>MPSYLSPGVYVEEVASGSRPIEGVGIEGVGTSVAAFVGLAPTGPLNEPTLVTNWTQYVAAFGDFTGGYYLAHSVYGFFNNGGSAAYVVRVGGSAEDAAADGSVNGAAAPAAVTGSTAKALPAAEPKQLGTFAVTATAAGQSGPLTVEVADPEGEGPAERFKLIVKDGDKPVETFDVSAKKGNRSYVVTQVKERSKLITVTEAAPSAQLVRPENQSLTLPAPPSAAPAVPAGQAESAHPGPAQYLGDSSDRTGFGGLEAIDEISMVAVPDLMAAYQRGAIDLEAVKAVQLGLIAHCELMGDRVAIIDPPPNQNARQIRVWRQETAGYDSKYAALYYPWIKSFDPATGQSRLVPPSGHVAGIWARNDSERGVHKAPANEVVRGAVDLELQITRGEQDLLNPIGVNCIRSFPGRGIRVWGARTLSSDPAWRYLNIRRYFNYLEESILIGTQWVVFEPNDHNLWARIRRNVSAFLVNEWRNGALFGQSPDQAYYVKCDEETNPPESVDLGRVVCEIGIAPVKPAEFVIFRLAQFSSGGGELDE[24x];>[24x]MSLPKPEDVLVAPNFGIQIDGVMVEYLNSVSNLQIEQDVIRYQQNQGTTGRNNVTLMPGVAKDGSVQVERGMSQSSVFTQWINDSMAGRMATARKNATIIVMDYEDNPVKRWNLRNAWCSKVVAGTLKAGDTNALTETITIVFEELVVE

In general, CIS are composed of a contractile sheath that surrounds an inner tube loaded with effectors, fitted with a baseplate complex. A conformational change in the baseplate complex triggers the contraction of the outer sheath, which leads to the propulsion of the inner tube into the target. Here we provide evidence that CIS from the model organism Streptomyces coelicolor (CISSc) function intracellularly and belong to a new class of CIS that exist as free-floating fully assembled particles in the cytoplasm and mediate cell death in response to stress conditions. Similar to the recently described sheath structures observed in AlgoCIS15 and tCIS19, the CISSc sheath is composed of a single protein, Cis2.

Different sets of two (IE), three (IEG) and five (IEGVG) amino acid residues were inserted into the N-terminal linker of Cis2 after position G25, resulting in the mutants CIS-N2, CIS-N3 and CIS-N5, respectively. For the CIS-N5 non-contractile mutant, more than 95% of the complexes were seen in the extended conformation. In vitro, the length of the CIS-N5 non-contractile mutant was homogeneous at ~230 nm. Next, we optimized the purification of CIS-N5 particles and performed cryo-EM. Helical reconstruction was used to generate an EM map, which we then used to build de novo the sheath-tube (Cis2-Cis1a) module in the extended conformation at 3.9 Å resolution. Domain 3 of the extended sheath (Cis2) was again too flexible to be resolved. The tube (Cis1a) structure and fold are highly similar to the tube structures already described for other CIS. The comparison of the sheath (domains 1/2) in the extended versus contracted states revealed an increase in diameter and shortening of the length upon contraction, similar to other CIS. The introduction of five extra amino acids in the CIS-N5 mutant induced conformational changes at the Cis2 N terminus, similar to a previous report.>[4x]VGA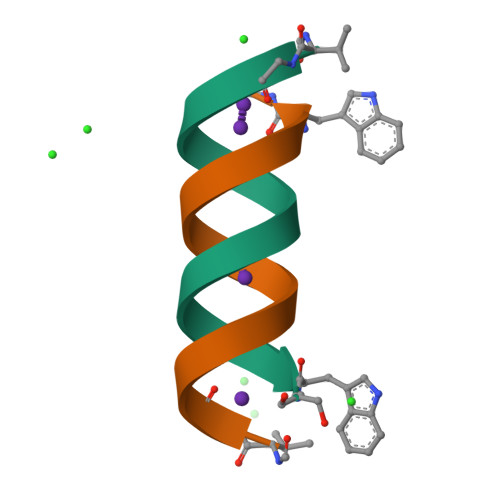LAVVVWLWLWLWX(2R)-2-benzyl-3-nitropropanoic acid | C10 H11 N O4 | 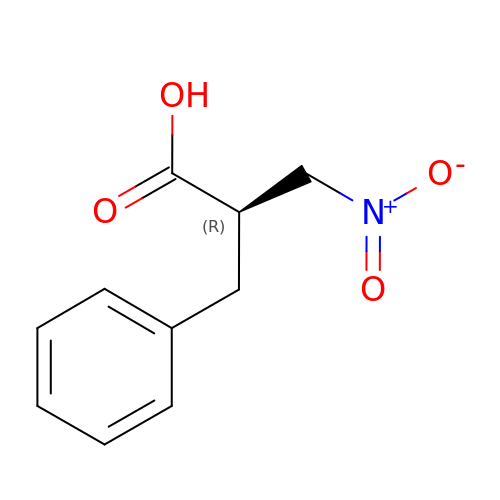GCXOTBPCUQHSAO-SECBINFHSA-N(phenylmethyl) 4-oxidanylpiperidine-1-carboxylate 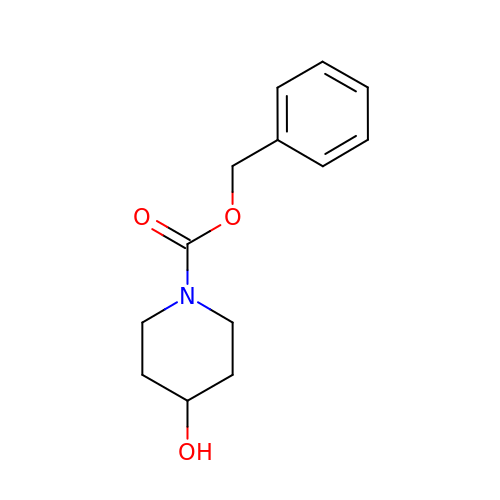| C13 H17 N O3 | JKIUUDJOCYHIGY-UHFFFAOYSA-N> STGSATTTPIDSLDDAYITPVQI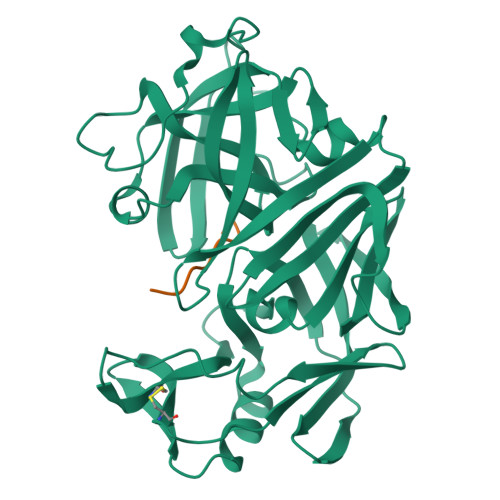GTPAQTLNLDFDTGSSDLWVFSSETTASEVDGQTIYTPSKSTTAKLLSGATWSISYGDGSSSSGDVYTDTVSVGGLTVTGQAVESAKKVSSSFTEDSTIDGLLGLAFSTLNTVSPTQQKTFFDNAKASLDSPVFTADLGYHAPGTYNFGFIDTTAYTGSITYTAVSTKQGFWEWTSTGYAVGSGTFKSTSIDGIADTGTTLLYLPATVVSAYWAQVSGAKSSSSVGGYVFPCSATLPSFTFGVGSARIVIPGDYIDFGPISTGSSSCFGGIQSSAGIGINIFGDVALKAAFVVFNGATTPTLGFASK;> HPFHLLVY>MPAHSFRIAAIPGDGIGLEVLPEGIRVLEAAALKHGLALEFDTFEWASCDYYLQHGKMMPDDWAEQLKQYDAIYFGAVGWPDKVPDHISLWGSLLKFRREFDQYVNIRPVRLFPGVPCALANRKVGDIDFVVVRENTEGEYSSLGGIMFENTENEIVIQESIFTRRGVDRILKYAFDLAEKRERKHVTSATKSNGMAISMPYWDKRTEAMAAHYPHVSWDKQHIDILCARFVLQPERFDVVVASNLFGDILSDLGPACAGTIGI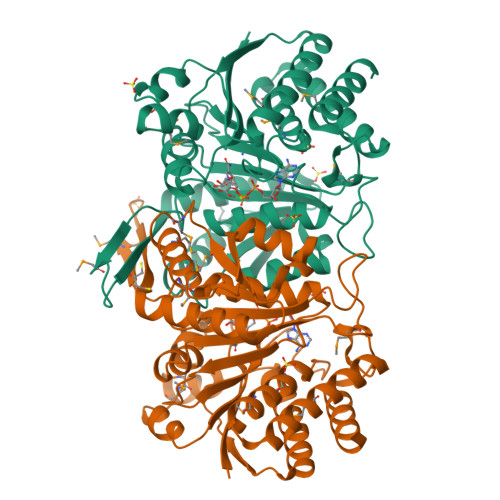APSANLNPERNFPSLFEPVHGSAPDIFGKNIANPIAMIWSGALMLEFLGQGDERYQRAHDDMLNAIERVIADGSVTPDMGGTLSTQQVGAAISDTLARLD[4x]> AALRERAGPVTWVMMIACVVVFIAMQILGDQEVMLWLAWPFDPTLKFEFWRYFTHALMHISLMHILFNLLWWWYLGGAVEKRLGSGKLIVITLISA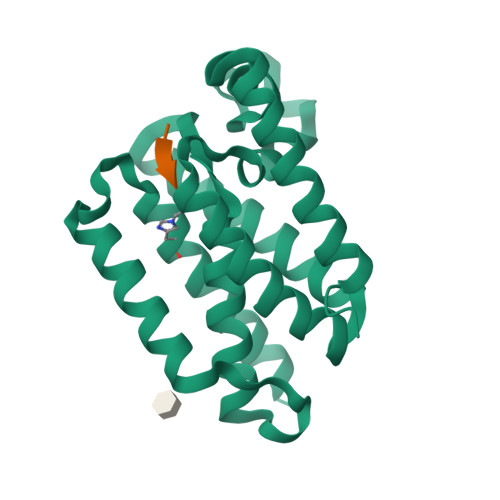LLSGYVQQKFSGPWFGGLSGVVYALMGYVWLRGERDPQSGIYLQRGLIIFALIWIVAGWFDLFGMSMANGAHIAGLAVGLAMAFVDSLNARKRKASLERENLYF> MVKIGVCGPVGSGKTALIEALTRHMSKDYDMAVITNDIYTKEDAEFMCKNSVMPRERIIGVETGGCPHTAIREDASMNLEAVEEMHGRFPNLELLLIESGGDNLSATFNPELADFTIFVIDVAEGDKIPRKGGPGITRSDLLVINKIDLAPYVGADLKVMERDSKKMRGEKPFIFTNIRAKEGLDDVIAWIKR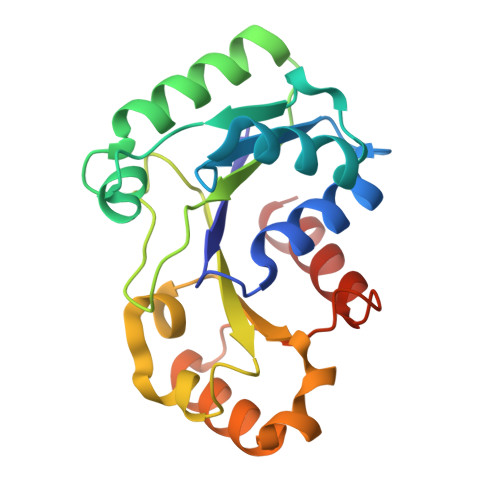NALLED>MAEAQVALDTNNDRSNHYSRPVFKQVLKVNSLQAQRVMERSFERVSNSLFSIDVILRIIGEQDEIDQVETVILEHISKVSEDLDKATAQLNKLMEDNGIDMM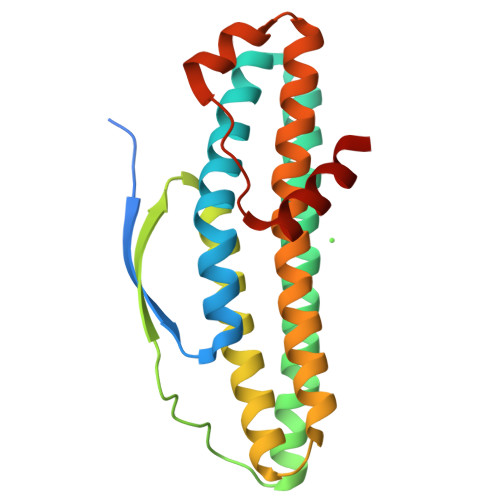PGYTNPNEYTIEINSPQVAQFAHLIRKLDTLMGIVDTLWLNTVLTSKQRTDATYQWQQRLIKLAGRIIGIEKRARISAHSKGKEGEVAEAAPESATGDKEIADEAEKTKAA[2x]> MGFDNLTDRLSRTLRNISGRGRLTEDNVKDTLREVRMALLEADVALPVVREFINRVKEKAVGHEVNKSLTPGQEFVKIVRNELVAAMGEENQTLNLAAQPPAVVLMAGLQGAGKTTSVGKLGKFLREKHKKKVLVVSADVYRPAAIKQLETLAEQVGVDFFPSDVGQKPVDIVNAALKEAKLKFYDVLLVDTAGRLHVDEAMMDEIKQVHASINPVETLFVVDAMTGQDAANTAKAFNEALPLTGVVLTKVDGDARGGAALSIRHITG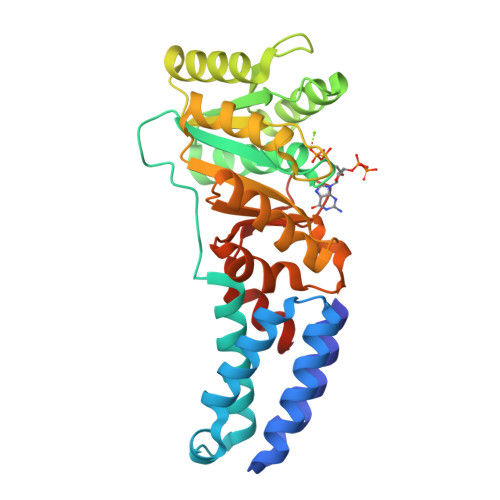KPIKFLGVGEKTEALEPFHPDRIASRILGMGDHHHHHH> AWDYDNNVIRGVNLGGWFVLEPYMTPSLFEPFQNGNDQSGVPVDEYHWTQTLGKEAASRILQKHWSTWITEQDFKQISNLGLNFVRIPIGYWAFQLLDNDP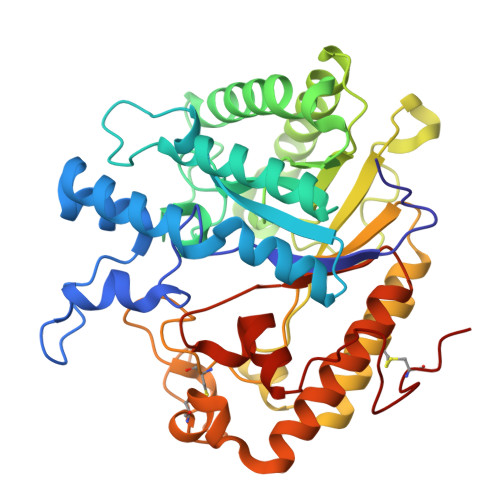YVQGQVQYLEKALGWARKNNIRVWIDLHGAPGSQNGFDNSGLRDSYNFQNGDNTQVTLNVLNTIFKKYGGNEYSDVVIGIELLNEPLGPVLNMDKLKQFFLDGYNSLRQTGSVTPVIIHDAFQVFGYWNNFLTVAEGQWNVVVDHHHYQVFSGGELSRNINDHISVACNWGWDAKKESHWNVAGEWSAALTDCAKWLNGVNRGARYEGAYDNAPYIGSCQPLLDISQWSDEHKTDTRRYIEAQLDAFEYTGGWVFWSWKTENAPEWSFQTLTYNGLFPQPVTDRQFPNQCGFH>[6x]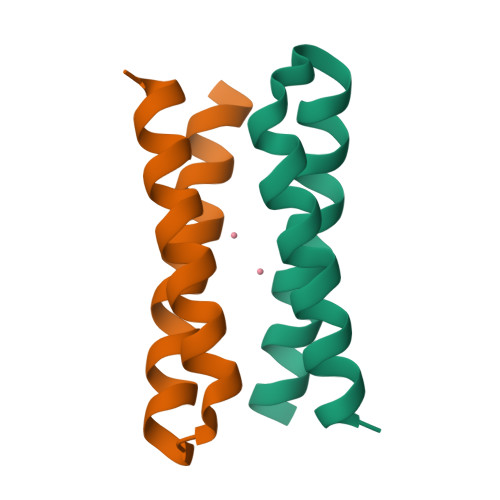XDYLRELLKLELQAIKQYREALEYVKLPVLAKILEDEEKHIEWLETILGX>[2x]MADAAPQLGKRKRELDVEEAHAASTEEKEAGVGNGTCAPVRLPFSGFRLQKVLRESARDKIIFLHGKVNEASGDGDGEDAVVILEKTPFQVEQVAQLLTGSPELQLQFSNDIYSTYHLFPPRQLNDVKTTVVYPATEKHLQKYLRQDLRLIRETGDDYRNITLPHLESQSLSIQWVYNILDKKAEADRIVFENPDPSDGFVLIPDLKWNQQQ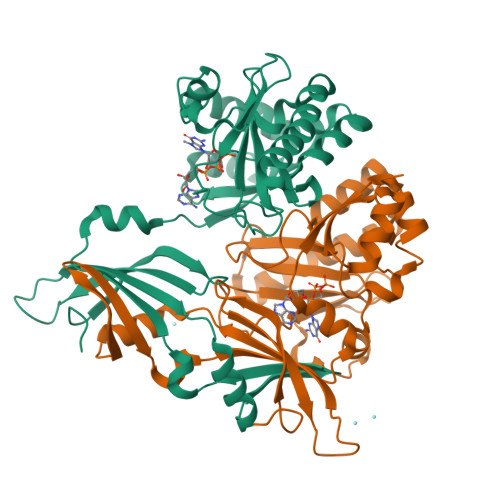LDDLYLIAICHRRGIRSLRDLTPEHLPLLRNILHQGQEAILQRYRMKGDHLRVYLHYLPSYYHLNVHFTALGFEAPGSGVERAHLLAEVIENLECDPRHYQQRTLTFALRADDPLLKLLQEAQQS> MGSHQERPLIGLLFSETGVTADIERSQRYGALLAVEQLNREGGVGGRPIETLSQDPGGDPDRYRLCAEDFIRNRGVRFLVGCYMSHTRKAVMPVVERADALLCYPNPYEGFEYSPNIVYGGPAPNQNSAPLAAYLIRHYGERVVFIGSDYIYPRESNHVMRHLYRQHGGTVLEEIYIPLYPSDDDLQRAVERIYQARADVVFSTVVGTGTAELYRAIARRYGDGRRPPIASLT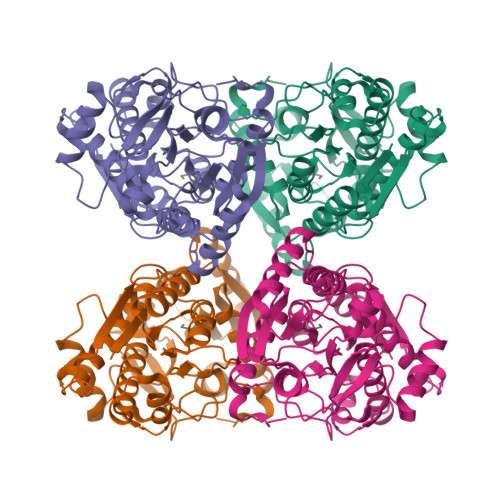TSEAEVAKMESDVAEGQVVVAPYFSSIDTPASRAFVQACHGFFPENATITAWAEAAYWQTLLLGRAAQAAGNWRVEDVQRHLYDIDIDAPQGPVRVERQNNHSRLSSRIAEIDARGVFQVRWQSPEPIRPDPYVVVHNLDDWSASMGGGPLP>[3x]QDLTVKMTDLQTGKPVGTIELSQNKYGVVFTPELADLTPGMHGFHIHQNGSCASSEKDGKVVLGGAAGGHYDPEHTNKHGFPWTDDNHKGDLPALFVSAN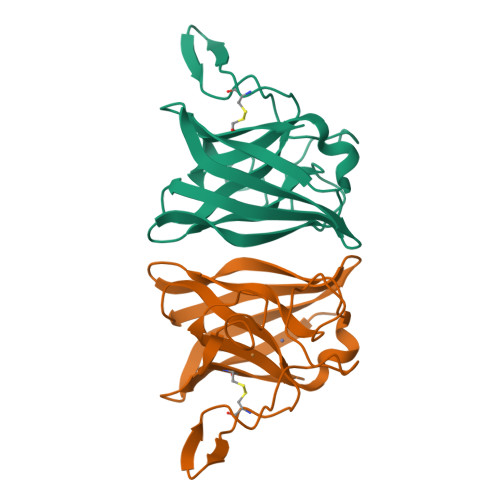GLATNPVLAPRLTLKELKGHAIMIHAGGDNHSDMPKALGGGGARVACGVIQ>[8x]GVALGAT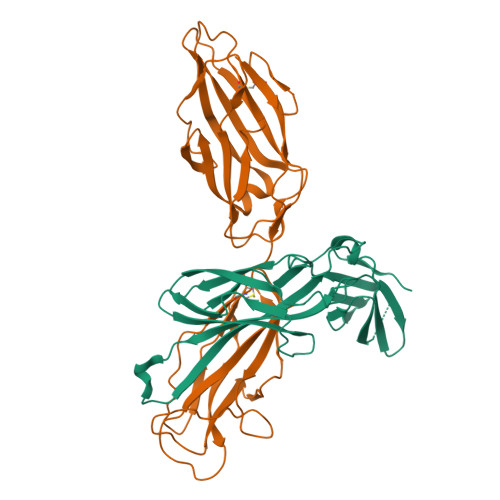RVIYPAGQKQVQLAVTNNDENSTYLIQSWVENADGVKDGRFIVTPPLFAMKGKKENTLRILDATNNQLPQDRESLFWMNVKAIPSMDKSKLTENTLQLAIISRIKLYYRPAKLALPPDQAAEKLRFRRSANSLTLINPTPYYLTVTELNAGTRVLENALVPPMGESAVKLPSDAGSNITYRTINDYGALTPKMTGVME;>FACKTANGTAIPIGGGSANVYVNLAPVVNVGQNLVVDLSTQIFCHNDYPETITDYVTLQRGSAYGGVLSNFSGTVKYSGSSYPFPTTSETPRVVYNSRTDKPWPVALYLTPVSSAGGVAIKAGSLIAVLILRQTNNYNSDDFQFVWNIYANNDVVVPTGGCDVSARDVTVTLPDYPGSVPIPLTVYCAKSQNLGYYLSGTTADAGNSIFTNTASFSPAQGVGVQLTRNGTIIPANNTVSLGAVGTSAVSLGLTANYARTGGQVTAGNVQSIIGVTFVYQ[8x]>GTSQVINGEMQFYARAKLFYQEVPATEEGMMGNFIELSSPDIQASQKFLRKFVGGPGRAGTDCALDCGSGIGRVSKHVLLPVFNSVELVDMMESFLLEAQNYLQVKGDKVESYHCYSLQEFTPPFRRYDVIWIQWVSGH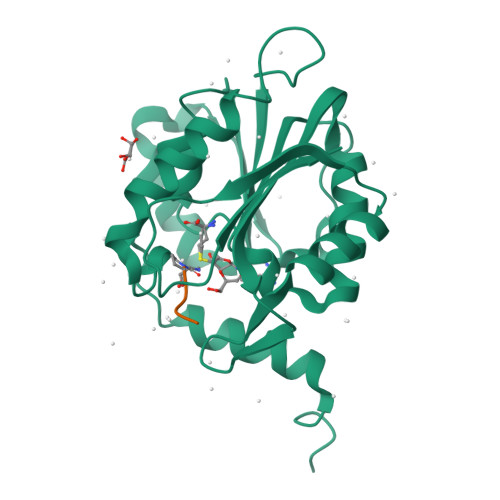LTDKDLLAFLSRCRDGLKENGIIILKDNVAREGCILDLSDSSVTRDMDILRSLIRKSGLVVLGQEKQDGFPEQCIPVWMFALH[2x];>[2x]XPKRIA> MAFAPIPRITWEHREVHLVQFHEPDIYNYSALLLSEDKDTLYIGAREAVFAVNALNISEKQHEVYWK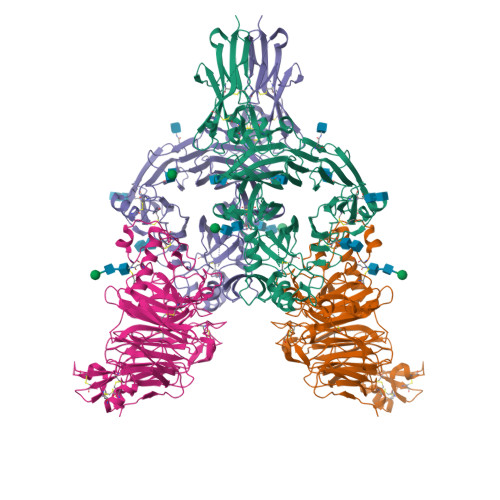VSEDKKAKCAEKGKSKQTECLNYIRVLQPLSATSLYVCGTNAFQPACDHLNLTSFKFLGKNEDGKGRCPFDPAHSYTSVMVDGELYSGTSYNFLGSEPIISRNSSHSPLRTEYAIPWLNEPSFVFADVIRKSPDSPDGEDDRVYFFFTEVSVEYEFVFRVLIPRIARVCKGDQGGLRTLQKKWTSFLKARLICSRPDSGLVFNVLRDVFVLRSPGLKVPVFYALFTPQLNNVGLSAVCAYNLSTAEEVFSHGKYMQSTTVEQSHTKWVRYNGPVPKPRPGACIDSEARAANYTSSLNLPDKTLQFVKDHPLMDDSVTPIDNRPRLIKKDVNYTQIVVDRTQALDGTVYDVMFVSTDRGALHKAISLEHAVHIIEETQLFQDFEPVQTLLLSSKKGNRFVYAGSNSGVVQAPLAFCGKHGTCEDCVLARDPYCAWSPPTATCVALHQTESPSRGLIQEMSGDASVCPDKSKGSYRQHFFKHGGTAELKCSQKSNLARVFWKFQNGVLKAESPKYGLMGRKNLLIFNLSEGDSGVYQCLSEERVKNKTVFQVVAKHVLEVKVVPKPVVAPTLSVVQTEGSRIATKVLVASTKHHHHHH;> ETGLQPLPPTAFTPNGTYLQHLARDPTSGTLYLGATNFLFQLSPGLQLEATVSTGPVLDSRDCLPPVMPDECPQAQPTNNPNQLLLVSPGALVVCGSVHQGVCEQRRLGQLEQLLLRPERPGDTQYVAANDPAVSTVGLVAQGLAGEPLLFVGRGYTSRGVGGGIPPITTRALWPPDPQAAFSYEETAKLAVGRLSEYSHHFVSAFARGASAYFLFLRRDLQAQSRAFRAYVSRVCLRDQHYYSYVELPLACEGGRYGLIQAAAVATSREVAHGEVLFAAFSSAAPPTVGRPPSAAAGASGASALCAFPLDEVDRLANRTRDACYTREGRAEDGTEVAYIEYDVNSDCAQLPVDTLDAYPCGSDHTPSPMASRVPLEATPILEWPGIQLTAVAVTMEDGHTIAFLGDSQGQLHRVYLGPGSDGHPYSTQSIQQGSAVSRDLTFDGTFEHLYVMTQSTLLKVPVASCAQHLDCASCLAHRDPYCGWCVLLGRCSRRSECSRGQGPEQWLWSFQPELGCLQGTKHHHHHH> EFAITSCPNNETVWETPIGVKYTLCPGSDYQNGGASLQTVRDIQSSLECAKICDSDARCNRAVYDNVNKACDVKNSTNPMQWAADDRFETIRLTNDLPEGAFISTCSFNETSYRVPETNAEYRICPDTDYTGVNAKVVEGVTTIQACAELCSNTQDCRKSVFDHINNACAIKAAEPATSIFWVQDKQFSTIRLPENIDPAVKGKWGDLIRLPVIPVAAYIVPSYPEPSRLLFFSSWSNDAFSGASGMTQFGDYDFATGAISQRTVTNTHHDMFCPGISQLEDGRILIQGGSDADTVSIYDPATNEFTRGPNMTLARGYQTSCTLSNGKVFTIGGAWSGERVGKNGEVYDPVANAWTYLPGADFRPMLTNDHEGIWREDNHAWLFGWKNGSIFQAGPSKDQHWYGIQGNGTVAKAATRDDDDAMCGVWVMYDAVAGKIFSAGGSPDYTDSPATQRAHITTIGEPNTPAEVERVADMGFPRGFANAVVLPDGQVLVTGGQRMSLVFTNTDGILVAELFNPETREWKQMAPMAVPRNYHSVSILLPDATVFSGGGGMCWVQNVGDSTAGCDKTVDHSDGEIFEPPYLFNEDGSRAARPVISAISADPIKAGATLTFTVEGVEGQG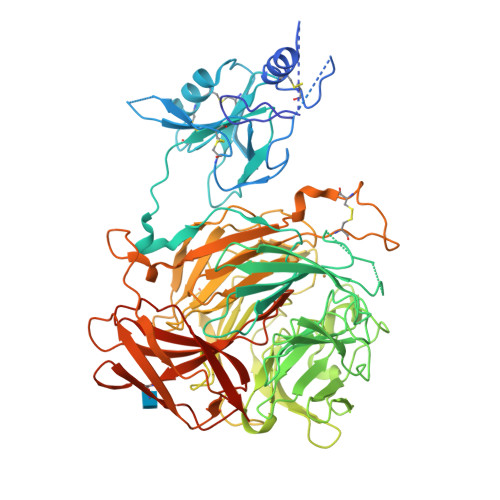TAALIRLGSVTHSVNSDQRRVPLNVTVSGNEYSATLPDDYGILLPGYYYLFVSTPQGTPSIAKTVHVILGLEQKLISEEDLNSAVDHHHHHH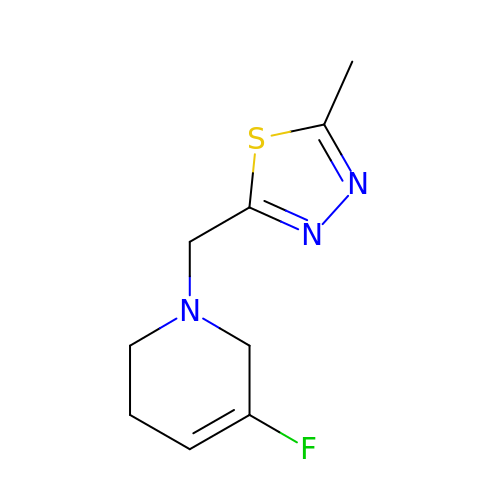5-fluoro-1-[(5-methyl-1,3,4-thiadiazol-2-yl)methyl]-1,2,3,6-tetrahydropyridine | C9 H12 F N3 S | WRJUIVWNZADJJL-UHFFFAOYSA-N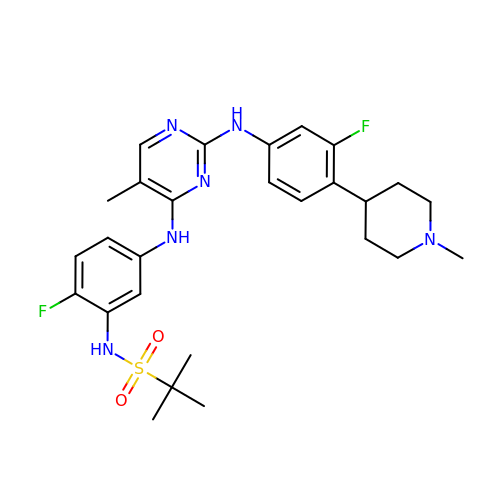N-{2-fluoro-5-[(2-{[3-fluoro-4-(1-methylpiperidin-4-yl)phenyl]amino}-5-methylpyrimidin-4-yl)amino]phenyl}-2-methylpropane-2-sulfonamide | C27 H34 F2 N6 O2 S | ACTFXTSBNQFCMD-UHFFFAOYSA-N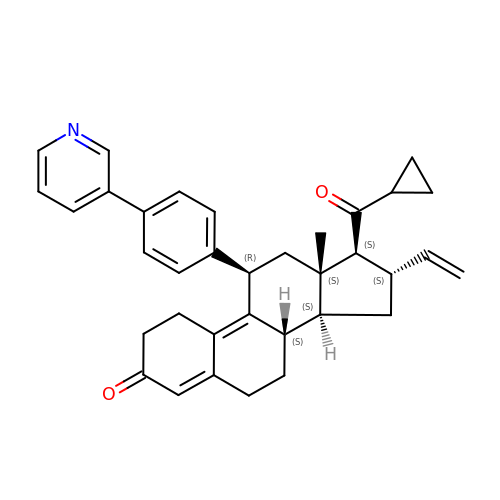(8S,11R,13S,14S,16S,17S)-17-cyclopropylcarbonyl-16-ethenyl-13-methyl-11-(4-pyridin-3-ylphenyl)-2,6,7,8,11,12,14,15,16,17-decahydro-1H-cyclopenta[a]phenanthren-3-one | C35 H37 N O2 | AUWGCRAJBXNPNU-WWVPXYRRSA-N>MSLQ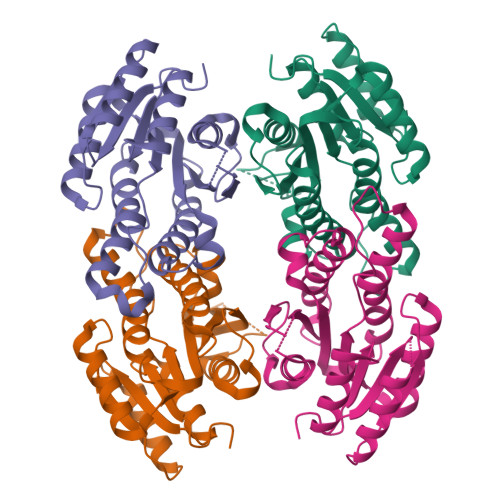RFTNRTIVVAGAGRDIGRACAIRFAQEGANVVLTYNGAAEGAATAVAEIEKLGRSALAIKADLTNAAEVEAAISAAADKFGEIHGLVHVAGGLIARKTIAEMDEAFWHQVLDVNLTSLFLTAKTALPKMAKGGAIVTFSSQAGRDGGGPGALAYATSKGAVMTFTRGLAKEVGPKIRVNAVCPGMISTTFHDTFTKPEVRERVAGATSLKREGSSEDVAGLVAFLASDDAAYVTGACYDINGGVLFSEGHHHHHH[4x]Stem-loop 5 (SL5, residues 150 to 294) contains the start codon of open reading frame 1a/b (ORF1a/b, residues 266 to 268). Additionally, phylogenetic covariance analysis and chemical probing experiments have shown that SL5′s secondary structure forms a four-way junction that sequesters the genome’s start codon within one of its helical stems. Beyond SARS-CoV-2, the multi-way junction and the sequestration of the start codon in a stem are conserved features across most coronaviruses, despite large sequence divergence from SARS-CoV-2 (average sequence identity of 51% for the NCBI Reference Sequences for alpha- and betacoronaviruses). SL5 has been proposed to play a role in protein–RNA or RNA–RNA binding because of its conserved hexaloops, characterized by 5′-UUYYGU-3′ (Y = C, U) repeat loop motifs.

First, we examined the SL5 domain from SARS-CoV-1 (residues 151 to 291, 143 nt, 46.1 kDa), which has high sequence similarity with SARS-CoV-2 (85.9% sequence identity) and also belongs to the Sarbecovirus subgenus. We found that SL5 of SARS-CoV-1 (7.0 Å resolution, 2.6 Å modeling convergence) adopts the same T-shaped fold and junction geometry as that of SARS-CoV-2, with an inter-helical angle of 86.8 ± 0.5° and distance between UUYYGU hexaloops of 82 ± 1 Å (N = 20). Additionally, we observed indications of other modes of flexibility that we did not model—for example, the SL5-stem in SARS-CoV-1. Despite this, after taking experimental uncertainty into account, we conclude that all betacoronavirus SL5s imaged exhibit interhelical angles within a narrow range, despite modeled and unmodeled flexibility.

> GGUUGACAAGAAACGAGUAACUCGUCCCUCUUCUGCAGACUGCUUACGGUUUCGUCCGUGUUGCAGUCGAUCAUCAGCAUACCUAGGUUUCGUCCGGGUGUGACCGAAAGGUAAGAUGGAGAGCCUUGUUCUUGGUGUCAACC(3R,5R)-7-[2-(4-fluorophenyl)-5-(1-methylethyl)-4-(morpholin-4-ylsulfonyl)-3-phenyl-1H-pyrrol-1-yl]-3,5-dihydroxyheptanoic acid | C30 H37 F N2 O7 S | 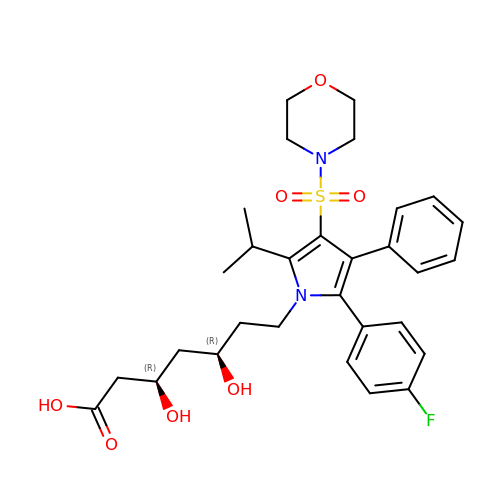XLVZRBHNHHAPDT-JWQCQUIFSA-N> ATFNIINNCPFTVWAAAVPGGGKRLDRGQNWIINPGAGTKGARVWPRTGCNFDGAGRGKCQTGDCNGLLQCQAFGQPPNTLAEYALNQFNNLDFFDISLVDGFNVAMEFSPTSGGCTRGIKCTADINGQCPNELRAPGGCNNPCTVFKTDQYCCNSGNCGLTNFSKFFKDRCP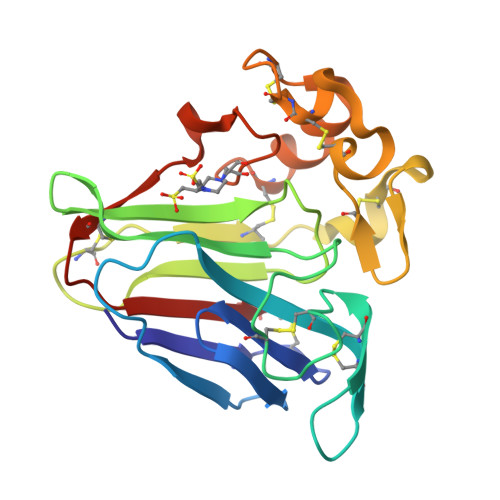DAYSYPKDDQTSTFTCPAGTNYKVVFCP>[2x]RSPWQGTLPPFLPCELQPHGLVNCNWLFLKSVPHFSAAAPRDNVTSLSLLSNRIHHLHDSDFAQLSNLQKLNLKWN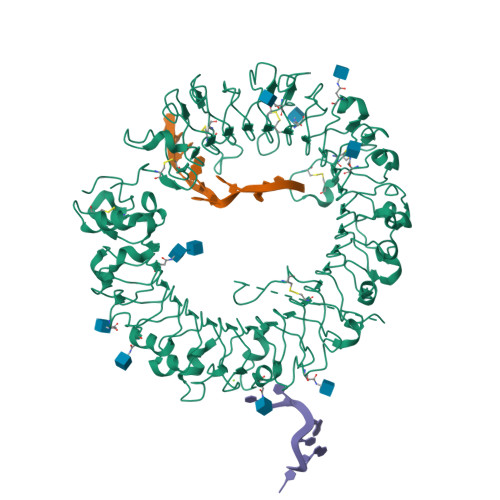CPPAGLSPMHFPCHMTIEPNTFLAVPTLEELNLSYNGITTVPALPSSLVSLILSRTNILQLDPTSLTGLHALRFLYMDGNCYYKNPCGRALEVAPGALLGLGNLTHLSLKYNNLTTVPRSLPPSLEYLLLSYNHIVTLAPEDLANLTALRVLDVGGNCRRCDHARNPCVECPHKFPQLHSDTFSHLSRLEGLVLKDSSLYQLNPRWFRGLGNLTVLDLSENFLYDCITKTKAFQGLAQLRRLNLSFNYHKKVSFAHLTLAPSFGSLLSLQELDMHGIFFRSLSQKTLQPLARLPMLQRLYLQMNFINQAQLGIFKDFPGLRYIDLSDNRISGAVEPVATTGEVDGGKKVWLTSRDLTPGPLDTPSSEDFMPSCKNLSFTLDLSRNNLVTVQPEMFAQLSRLQCLRLSHNSISQAVNGSQFVPLTSLQVLDLSHNKLDLYHGRSFTELPRLEALDLSYNSQPFSMRGVGHNLSFVAQLPTLRYLSLAHNGIHSRVSQQLCSTSLWALDFSGNSLSQMWAEGDLYLRFFQGLRSLIRLDLSQNRLHTLLPCTLGNLPKSLQLLRLRNNYLAFFNWSSLTLLPNLETLDLAGNQLKALSNGSLPSGTQLQRLDVSRNSIIFVVPGFFALATRLRELNLSANALRTVEPSWFGFLAGSLEVLDVSANPLHCACGAAFVDFLLQVQAAVPGLPSRVKCGSPGQLQGRSIFAQDLRLCLDESLSWDEFLVPR>MSQTETSHSGYIDFKKESQPSVFQCKKCFQIVGDSNAWVISHREYLSFTLSDAVENSVRVEDTFKRSDDGLCVYSELSCTRCNEVIGKVYNSTPIYLDDIRDMYTFSMDKLQAYQLGNK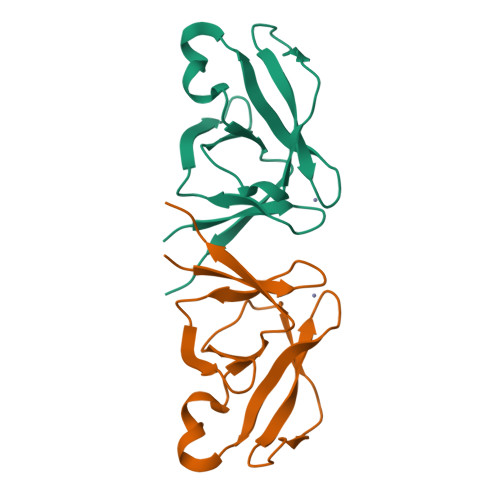T[3x]> RRALRLGVNGLPNSLEPVNAISNVGPRIVNQIFDTLIARDFFAKGAPGNAIDLVPALAESWERIDEKSVRFKLRQKVMFHDGVELTADDVAYTFSSERLWGPEAIKKIPLGKSYSLDFDEPVVEDKYTVTLRTKTPSYLIETFVASWMSRIVPKEYYKKLGAVDFGNKPVGTGPYKFVEFVAGDRVVLEANDAYWGPKPTASKITYQIVAEPATRVAGLI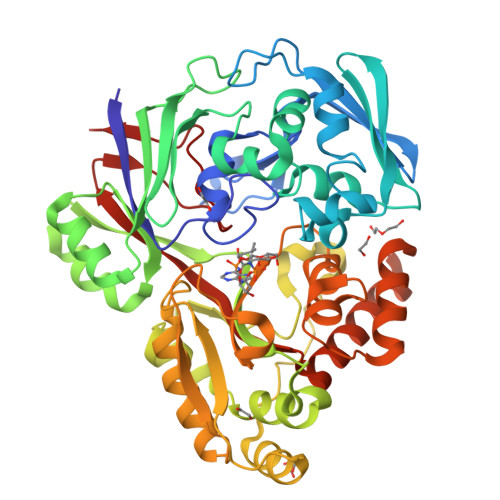SGEYDIITTLTPDDIQLINSYPDLETRGTLIENFHMFTFNMNQEVFKDKKLRRALALAVNRPIMVEALWKKQASIPAGFNFPNYGETFDPKRKAMEYNVEEAKRLVKESGYDGTPITYHTMGNYYANAMPALMMMIEMWKQIGVNVVMKTYAPGSFPPDNQTWMRNWSNGQWMTDAYATIVPEFGPNGQVQKRWGWKAPAEFNELCQKVTVLPNGKERFDAYNRMRDIFEEEAPAVILYQPYDVYAARKDVHWKPVSFEMMEFRNNLSFG> MFYIDNDSGVTVMPPVSAQRSAIVRWFSEGDGNNVITWPGMDWFNIVQAELLNTLEEAGIQPDKTKLNQLALSIKAIMSNNALLIKNNLSEIKTAGASAQRTARENLDIYDASLNKKGLVQLTSATDSPSETLAATAKAVKIAMDNANARLAKDRNGADIPNKPLFIQNLGLQETVNQASGALQQNQNGADIPGKDTFTKNIGACRAYSAWLNIGGDSQVWTTAQFISWLESQGAFNHPYWMCKGSWAYANNKVITDTGCGNICLAGAVVEVIGTRGAMTIRVTTPSTSSGGGITNAQFTYINHGDAYAPGWRRDYNTKNQQPAFALGQTGSTVGNDKAVGWNWNSGVYNANIGGASTLILHFNMNTGSCPAVQFRVNYRNGGIFYRSARDGYGFEADWSEIYTTTRKPSAGDVGAYTQAECNSRFI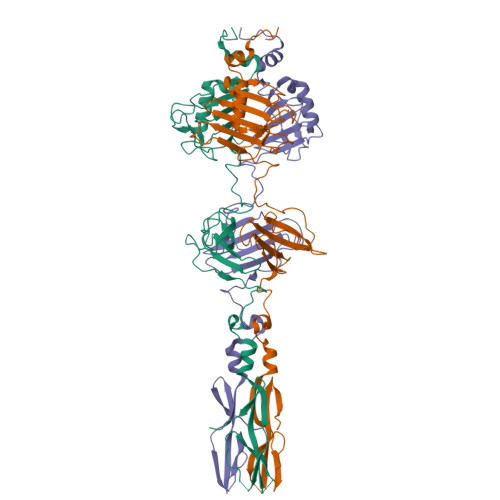TGIRLGGLSSVQTWNGPGWSDRSGYVVTGSVNGNRDELIDTTQARPIQYCINGTWYNAGSI> SVAILQKRDHEGFGFVLRGAKAETPI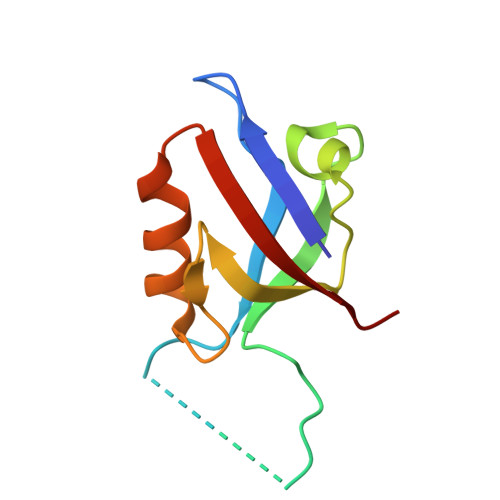EEFTPTPAFPALQYLESVDVEGVAWKAGLRTGDFLIEVNGVNVVKVGHKQVVGLIRQGGNRLVMKVVSVT>ARKCSLTGKWTDDLGSNMTIGAVNSRGEFTGTYITAVADNPGNITLSPLLGIQHKRAS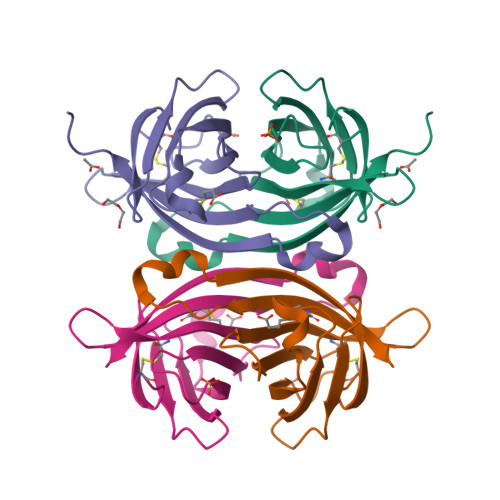QPTFGFTVNWKFSESTTVFTGQCFIDRNGKEVLKTMWLLRSSVNDISDDWIATRVGINIFTRQRTQK[2x]>[2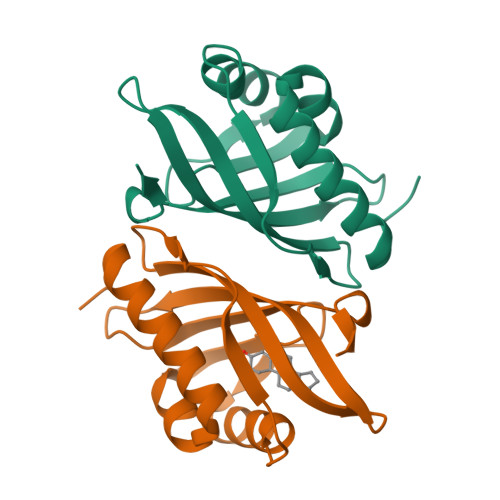x]MNLPTAQEVQGLMARYIELVDVGDIEAIVQMYADDATVEDPFGQPPIHGREQIAAFYRQGLGGGKVRACLTGPVRASHNGCGAMPFRVEMVWNGQPCALDVIDVMRFDEHGRIQTMQAYWSEVNLSVREPQLVPR>[8x]SVRSSSRTPSDKPVAHVVANPQAEGQLQWLNRRANALLANGVELRDNQLVVPSEGLYLIYSQVLFKGQGCPSTHVLLTHTISRIAVSYQTKVNLLSAIKSPCQRETPE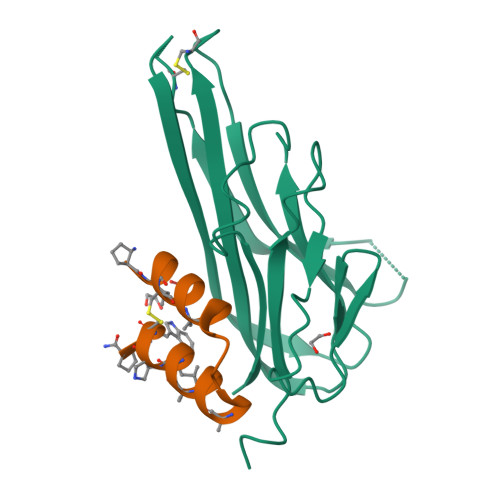GAEAKPWYEPIYLGGVFQLEKGDRLSAEINRPDYLDFAESGQVYFGIIAL;>[8x]XLGWCIGEAGTDPNLNHAQFRAKILXCWX1-{[(5R,6S)-5,6-bis(4-chlorophenyl)-6-methyl-3-(propan-2-yl)-5,6-dihydroimidazo[2,1-b][1,3]thiazol-2-yl]carbonyl}-N,N-dimethyl-L-prolinamide 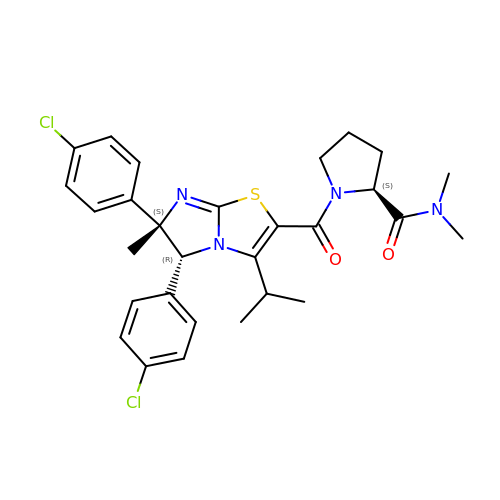| C29 H32 Cl2 N4 O2 S | BWUMOCARMRPCIP-HQQGYVGFSA-N> CCTCGCTCTC;> G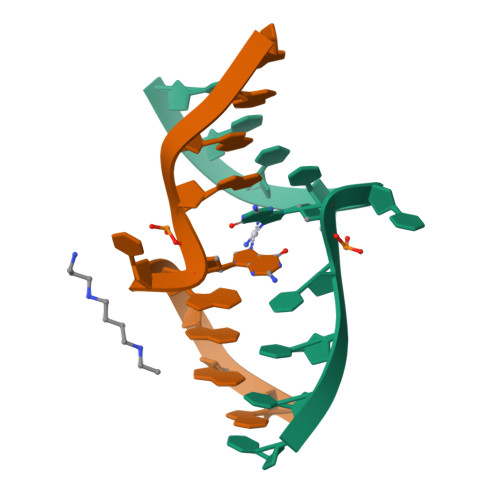AGAGCGAGG>MFNNEPLEQIDKELHDILADEEKRQRETINLIASENLTNGAVRECLGNRVSNKYSEGYPKKRYYGGNDFIDKIEELCQKRALEAFNVSDEEWGVNVQPLSGSAANVQALYALVGVKGKIMGMHLCSGGHLTHGFFDEKKKVSITSDMFESKLYKCNSQGYVDLDAVREMALSFKPKVIICGYTSYPRDIDYQQFRQICDEVNAYLFADISHISSFVACNILNNPFLHADVVTTTTHKILRGPRSALIFFNKKRNPGIEQKINSAVFPSFQGGPHNNKIAAVACQLKEVHSPAFKEYTQQVLLNSKALAKALISKQIDLVTNGTDNHLIVVDLRKFSITGSKLQETCNAINVSLNKNTIPSDVDAVSPSGVRIGTPAMT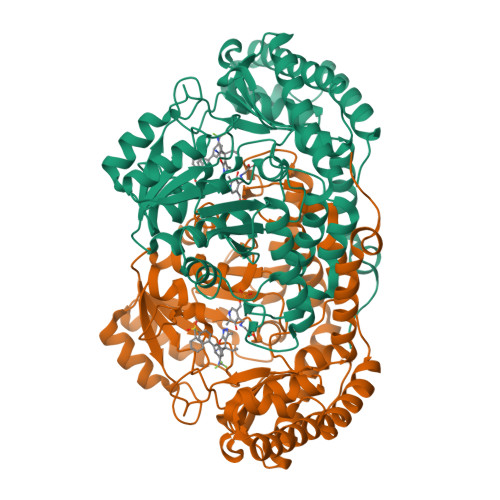TRGAKEKDMEFIADVLARAIKITVDLQEQYGKKLVDFKKGLPGNAQLQQLKQEVVTWAGALPFP[3x]> MLRESFAISGDSLISLASTGKRVPIKDLLGEKDFEIWAINEQTMKLESAKVSRVFCTGKKLVYTLKTRLGRTIKATANHRFLTIDGWKRLDELSLKEHIALPRKL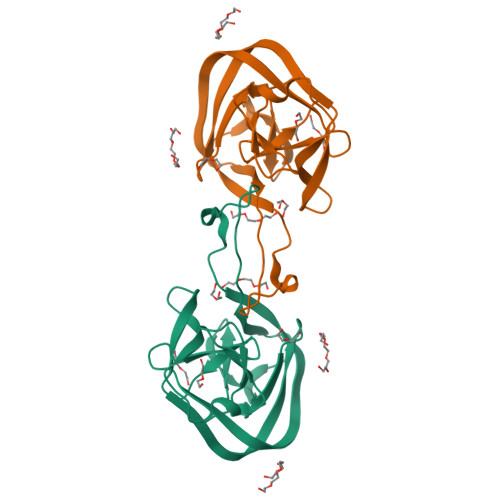ESSSLQLAPEIEKLPQSDIYWDPIVSITETGVEEVFDLTVPGLRNFVANDIIVHASIEQDKLGG>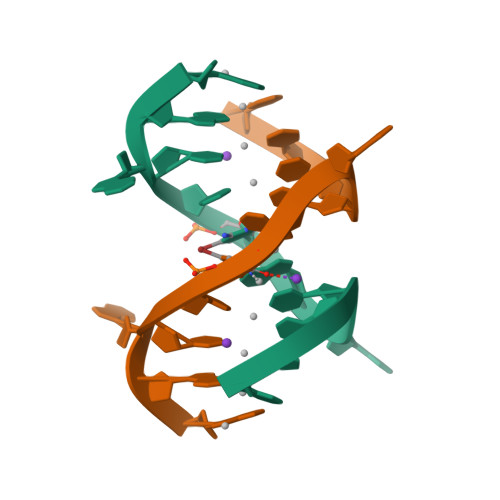 GGACTCGACTCC>[3x]MAGAIENARKEIKRISLEDHAESEYGAIYSVSGPVVIAENMIGCAMYELVKVGHDNLVGEVIRIDGDKATIQVYEETAGLTVGDPVLRTGKPLSVELGPGLMETIYDGIQRPLKAIKEESQSIYIPRGIDTPALDRTIKWQFTPGKFQVGDHISGGDIYGSVFENSLISSHKILLPPRSRGTITWIAPAGEYTLDEKILEVEFDGKKSDFTLYHTWPVRVPRPVTEKLSADYPLLTGQRVLDALFPCVQGGTTCIPGAFGCGKTVISQSLSKYSNSD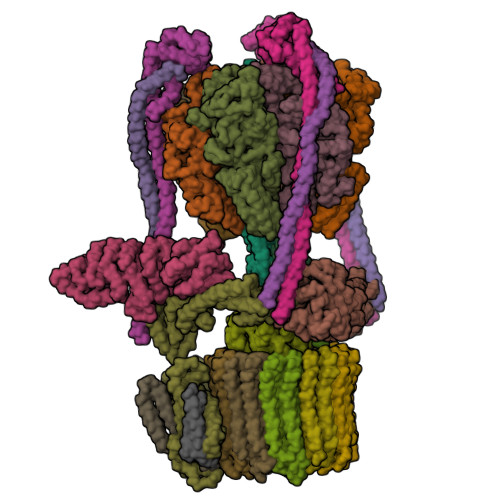AIIYVGCGERGNEMAEVLMEFPELYTEMSGTKEPIMKRTTLVANTSNMPVAAREASIYTGITLAEYFRDQGKNVSMIADSSSRWAEALREISGRLGEMPADQGFPAYLGAKLASFYERAGKAVALGSPDRTGSVSIVAAVSPAGGDFSDPVTTATLGITQVFWGLDKKLAQRKHFPSINTSVSYSKYTNVLNKFYDSNYPEFPVLRDRMKEILSNAEELEQVVQLVGKSALSDSDKITLDVATLIKEDFLQQNGYSTYDAFCPIWKTFDMMRAFISYHDEAQKAVANGANWSKLADSTGDVKHAVSSSKFFEPSRGEKEVHGEFEKLLSTMQERFAESTDDYKDHDGDYKDHDIDYKDDDDK;>MVLSDKELFAINKKAVEQGFNVKPRLNYNTVSGVNGPLVILEKVKFPRYNEIVNLTLPDGTVRQGQVLEIRGDRAIVQVFEGTSGIDVKKTTVEFTGESLRIPVSEDMLGRIFDGSGRPIDNGPKVFAEDYLDINGSPINPYARIYPEEMISTGVSAIDTMNSIARGQKIPIFSASGLPHNEIAAQICRQAGLVRPTKDVHDGHEENFSIVFAAMGVNLETARFFKQDFEENGSLERTSLFLNLANDPTIERIITPRLALTTAEYLAYQTERHVLTILTDMSSYADALREVSAAREEVPGRRGYPGYMYTDLSTIYERAGRVEGRNGSITQIPILTMPNDDITHPIPDLTGYITEGQIFVDRQLHNKGIYPPINVLPSLSRLMKSAIGEGMTRKDHGDVSNQLYAKYAIGKDAAAMKAVVGEEALSIEDKLSLEFLEKFEKTFITQGAYEDRTVFESLDQAWSLLRIYPKEMLNRISPKILDEFYDRARDDADEDEEDPDTRSSGKKKDASQEESLI[3x];>MSSAITALTPNQVNDELNKMQAFIRKEAEEKAKEIQLKADQEYEIEKTNIVRNETNNIDGNFKSKLKKAMLSQQITKSTIANKMRLKVLSAREQSLDGIFEETKEKLSGIANNRDEYKPILQSLIVEALLKLLEPKAIVKALERDVDLIESMKDDIMREYGEKAQRAPLEEIVISNDYLNKDLVSGGVVVSNASDKIEINNTLEERLKLLSEEALPAIRLELYGPSKTRKFFD[3x];>MSQKNGIATLLQAEKEAHEIVSKARKYRQDKLKQAKTDAAKEIDSYKIQKDKELKEFEQKNAGGVGELEKKAEAGVQGELAEIKKIAEKKKDDVVKILIETVIKPSAEVHINAL[3x];> MSGNREQVFPTRMTLGLMKTKLKGANQGYSLLKRKSEALTKRFRDITKRIDDAKQKMGRVMQTAAFSLAEVSYATGENIGYQVQESVSTARFKVRARQENVSGVYLSQFESYIDPEINDFRLTGLGRGGQQVQRAKEIYSRAVETLVELASLQTAFIILDEVIKVTNRRVNAIEHVIIPRTENTIAYINSELDELDREEFYRLKKVQEKKQNETAKLDAEMKLKRDRAEQDASEVAADEEPQGETLVADQEDDVIF;> MAEKRTLIAVIADEDTTTGLLLAGIGQITPETQEKNFFVYQEGKTTKEEITDKFNHFTEERDDIAILLINQHIAENIRARVDSFTNAFPAILEIPSKDHPYDPEKDSVLKRVRKLFGE;> MATALYTANDFILISLPQNAQPVTAPGSKTDSWFNETLIGGRAFVSDFKIPEFKIGSLDTLIVESEELSKVDNQIGASIGKIIEILQGLNETSTNAYRTLPINNMPVPEYLENFQWQTRKFKLDKSIKDLITLISNESSQLDADVRATYANYNSAKTNLAAAERKKTGDLSVRSLHDIVKPEDFVLNSEHLTTVLVAVPKSLKSDFEKSYETLSKNVVPASASVIAEDAEYVLFNVHLFKKNVQEFTTAAREKKFIPREFNYSEELIDQLKKEHDSAASLEQSLRVQLVRLAKTAYVDVFINWFHIKALRVYVESVLRYGLPPHFNIKIIAVPPKNLSKCKSELIDAFGFLGGNAFMKDKKGKINKQDTSLHQYASLVDTEYEPFVMYIINL;> MGATKILMDSTHFNEIRSIIRSRSVAWDALARSEELSEIDASTAKALESILVKKNIGDGLSSSNNAHSGFKVNGKTLIPLIHLLSTSDNEDCKKSVQNLIAELLSSDKYGDDTVKFFQEDPKQLEQLFDVSLKGDFQTVLISGFNVVSLLVQNGLHNVKLVEKLLKNNNLINILQNIEQMDTCYVCIRLLQELAVIPEYRDVIWLHEKKFMPTLFKILQRATDSQLATRIVATNSNHLGIQLQYHSLLLIWLLTFNPVFANELVQKYLSDFLDLLKLVKITIKEKVSRLCISIILQCCSTRVKQHKKVIKQLLLLGNALPTVQSLSERKYSDEELRQDISNLKEILENEYQELTSFDEYVAELDSKLLCWSPPHVDNGFWSDNIDEFKKDNYKIFRQLIELLQAKVRNGDVNAKQEKIIIQVALNDITHVVELLPESIDVLDKTGGKADIMELLNHSDSRVKYEALKATQAIIGYTFK;> MNQEEAIFRSADMTYVQLYIPLEVIREVTFLLGKMSVFMVMDLNKDLTAFQRGYVNQLRRFDEVERMVGFLNEVVEKHAAETWKYILHIDDEGNDIAQPDMADLINTMEPLSLENVNDMVKEITDCESRARQLDESLDSLRSKLNDLLEQRQVIFECSKFIEVNPGIAGRATNPEIEQEERDVDEFRMTPDDISETLSDAFSFDDETPQDRGALGNDLTRNQSVEDLSFLEQGYQHRYMITGSIRRTKVDILNRILWRLLRGNLIFQNFPIEEPLLEGKEKVEKDCFIIFTHGETLLKKVKRVIDSLNGKIVSLNTRSSELVDTLNRQIDDLQRILDTTEQTLHTELLVIHDQLPVWSAMTKREKYVYTTLNKFQQESQGLIAEGWVPSTELIHLQDSLKDYIETLGSEYSTVFNVILTNKLPPTYHRTNKFTQAFQSIVDAYGIATYKEINAGLATVVTFPFMFAIMFGDMGHGFILFLMALFLVLNERKFGAMHRDEIFDMAFTGRYVLLLMGAFSVYTGLLYNDIFSKSMTIFKSGWQWPSTFRKGESIEAKKTGVYPFGLDFAWHGTDNGLLFSNSYKMKLSILMGYAHMTYSFMFSYINYRAKNSKVDIIGNFIPGLVFMQSIFGYLSWAIVYKWSKDWIKDDKPAPGLLNMLINMFLAPGTIDDQLYSGQAKLQVVLLLAALVCVPWLLLYKPLTLRRLNKNGGGGRPHGYQSVGNIEHEEQIAQQRHSAEGFQGMIISDVASVADSINESVGGGEQGPFNFGDVMIHQVIHTIEFCLNCISHTASYLRLWALSLAHAQLSSVLWDMTISNAFSSKNSGSPLAVMKVVFLFAMWFVLTVCILVFMEGTSAMLHALRLHWVEAMSKFFEGEGYAYEPFSFRAIIE;> MVFGQLYALFIFTLSCCISKTVQADSSKESSSFISFDKESNWDTISTISSTADVISSVDSAIAVFEFDNFSLLDNLMIDEEYPFFNRFFANDVSLTVHDDSPLNISQSLSPIMEQFTVDELPESASDLLYEYSLDDKSIVLFKFTSDAYDLKKLDEFIDSCLSFLEDKSGDNLTVVINSLGWAFEDEDGDDEYATEETLSHHDNNKGKEGDDDILSSIWTEGLLMCLIVSALLLFILIVALSWISNLDITYGALEKSTNPIKKNN;> MNKESKDDDMSLGKFSFSHFLYYLVLIVVIVYGLYKLFTGHGSDINFGKFLLRTSPYMWANLGIALCVGLSVVGAAWGIFITGSSMIGAGVRAPRITTKNLISIIFCEVVAIYGLIIAIVFSSKLTVATAENMYSKSNLYTGYSLFWAGITVGASNLICGIAVGITGATAAISDAADSALFVKILVIEIFGSILGLLGLIVGLLMAGKASEFQ;> MEGVYFNIDNGFIEGVVRGYRNGLLSNNQYINLTQCDTLEDLKLQLSSTDYGNFLSSVSSESLTTSLIQEYASSKLYHEFNYIRDQSSGSTRKFMDYITYGYMIDNVALMITGTIHDRDKGEILQRCHPLGWFDTLPTLSVATDLESLYETVLVDTPLAPYFKNCFDTAEELDDMNIEIIRNKLYKAYLEDFYNFVTEEIPEPAKECMQTLLGFEADRRSINIALNSLQSSDIDPDLKSDLLPNIGKLYPLATFHLAQAQDFEGVRAALANVYEYRGFLETGNLEDHFYQLEMELCRDAFTQQFAISTVWAWMKSKEQEVRNITWIAECIAQNQRERINNYISVY;> MSSFYTVVGVFIVVSAMSVLFWIMAPKNNQAVWRSTVILTLAMMFLMWAITFLCQLHPLVAPRRSDLRPEFAE;> MRPVVSTGKAWCCTVLSAFGVVILSVIAHLFNTNHESFVGSINDPEDGPAVAHTVYLAALVYLVFFVFCGFQVYLARRKPSIELR;>MTELCPVYAPFFGAIGCASAIIFTSLGAAYGTAKSGVGICATCVLRPDLLFKNIVPVIMAGIIAIYGLVVSVLVCYSLGQKQALYTGFIQLGAGLSVGLSGLAAGFAIGIVGDAGVRGSSQQPRLFVGMILILIFAEVLGLYGLIVALLLNSRATQDVVC[8x];> MSTQLASNIYAPLYAPFFGFAGCAAAMVLSCLGAAIGTAKSGIGIAGIGTFKPELIMKSLIPVVMSGILAIYGLVVAVLIAGNLSPTEDYTLFNGFMHLSCGLCVGFACLSSGYAIGMVGDVGVRKYMHQPRLFVGIVLILIFSEVLGLYGMIVALILNTRGSE> FEKHGTYYEIFVRSFYDSDGDGIGDLKGIIEKLDYLNDGDPETIADLGVNGIWLMPIFKSPSYHGYDVTDYYKINPDYGTLEDFHKLVEAAHQRGIKVIIDLPINHTSERHPWFLKASRDKNSEYRDYYVWAGPDTDTKETKLDGGRVWHYSPTGMYYGYFWSGMPDLNYNNPEVQEKVIGIAKYWLKQGVDGFRLDGAMHIFPPAQYDKNFTWWEKFRQEIEEVKPVYLVGEVWDISETVAPYFKYGFDSTFNFKLAEAVIATAKAGFPFGFNKKAKHIYGVYDREVGFGNYIDAPFLTNHDQNRILDQLGQDRNKARVAASIYLTLPGNPFIYYGEEIGMRGQGPHEVIREPFQWYNGSGEGETYWEPAMYNDGFTSVEQEEKNLDSLLNHYRRLIHFRNENPVFYTGKIEIINGGLNVVAFRRYNDKRDLYVYHNLVNRPVKIKVASGNWTLLFNSGD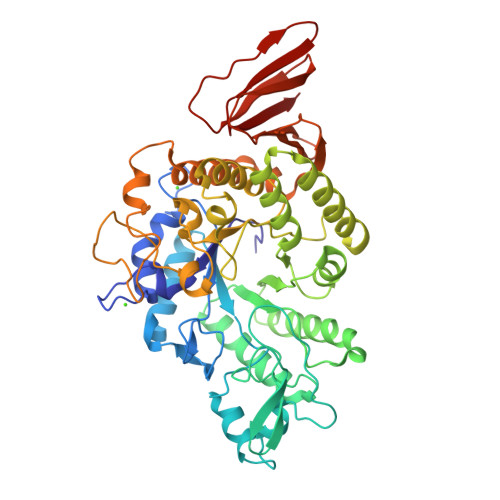KEITPVEDNNKLMYTIPAYTTIVLEKE>[4x]AMADTIV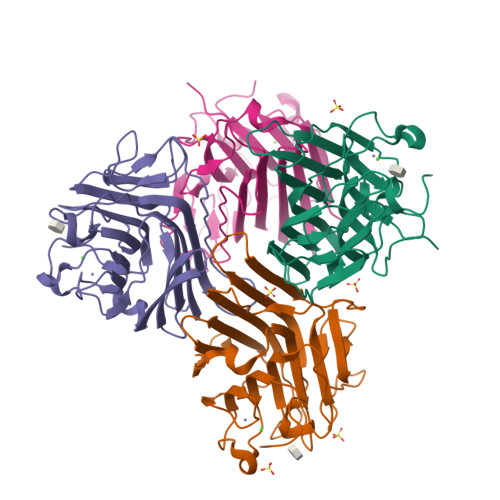AVELDSYPNTDIGDPNYPHIGIDIKSIRSKSTARWNMQTGKVGTVHISYNSVAKRLSAVVSYSGSSSTTVSYDVDLNNVLPEWVRVGLSATTGLYKETNTILSWSFTSKLKTNSIADENSLHFSFHKFSQNPKDLILQGDAFTDSDGNLQLTKVSSSGDPQGNSVGRALFYAPVHIWEKSAVVASFDATFTFLIKSPDREPADGITFFIANTDTSIPSGSGGRLLGLFPDAN> MVKQIESKTAFQEALDAAGDKLVVV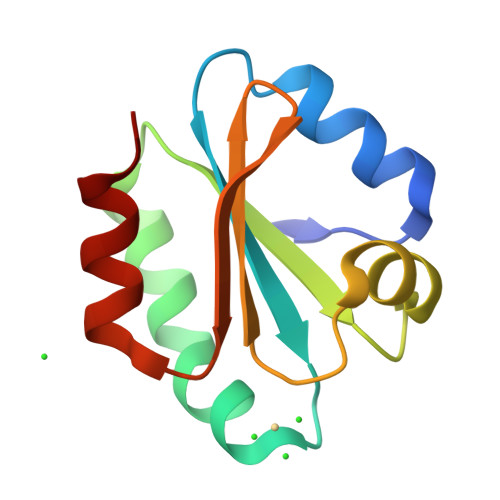DFSATWCGPSKMIKPFFHSLSEKYSNVIFLEVDVDDSQDVASESEVKSMPTFQFFKKGQKVGEFSGANKEKLEATINELV> MSSEANPPVLEPFTVTVVDRNVKHQVEGEPEEEGHPDHEVQGVMFATNVKYIFEDDQELLPE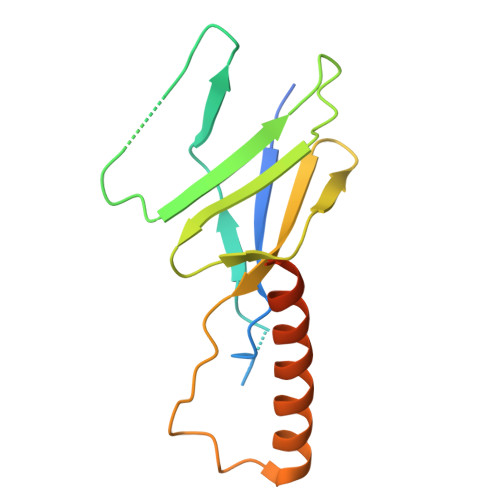QEDPAIENVVIIEADESLRVTQVEMISDQFKQVGYEVRDGNEVCIDAMSRFETPRQLGNLPLEKLVQLYKLQNDQLHSLFNTLAGQFYLNAHHHHHH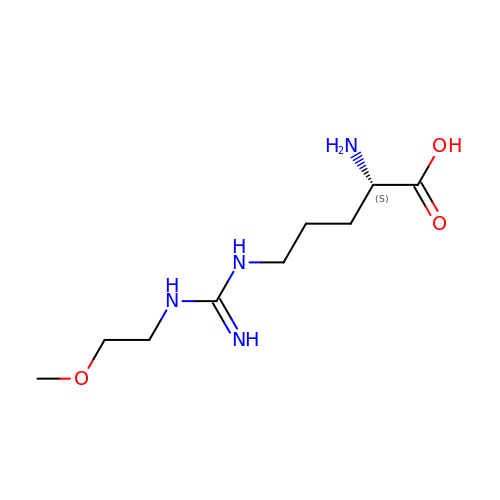N~5~-{IMINO[(2-METHOXYETHYL)AMINO]METHYL}-L-ORNITHINE | C9 H20 N4 O3 | XMBSMMCPKFDGEO-ZETCQYMHSA-N Here, we reveal the structure, binding and cleavage of moxalactam antibiotic bound to L1 metallo-β-lactamase (MBL) from Stenotrophomonas maltophilia. The structure of L1 from S. maltophilia adopts a typical MBL fold with two β sheets decorated with exposed α-helices and loops. The zinc ions are coordinated by H116, H118 and H196 (termed Zn1) and D120, H121 and H263 (termed Zn2). The L1 uses two-zinc scaffold that is central to MBL’s activity, contributing to active site stability, substrate binding, and catalysis.

The electron density for the hydrolyzed moxalactam continued to be visible in the 300, 500, 2000, and 4000 ms time points. After the bond scission occurs between C-8 and N-5 atoms there are some significant distance changes, and the product settles down by binding to two zinc ions and stays bound till 4000 ms time point. Then the ring rotates back clockwise from 500 to 4000 ms and returns to the configuration similar to that of the intact substrate. The product is then stabilized and stays bound to both zinc ions.

> SNAASAAEAPLPQLRAYTVDASWLQPMAPLQVADHTWQIGTEDLTALLVQTAEGAVLLDGGMPQMAGHLLDNMKLRGVAPQDLRLILLSHAHADHAGPVAELKRRTGAHVAANAETAVLLARGGSNDLHFGDGITYPPASADRIIMDGEVVTVGGIAFTAHFMPGHTPGSTAWTWTDTRDGKPVRIAYADSLSAPGYQLKGNPRYPRLIEDYKRSFATVRALPCDLLLTPHPGASNWNYAVGSKASAEALTCNAYADAAEKKFDAQLARETAGTR> KMSDLRTVTLYKGKAGFGFSLLGP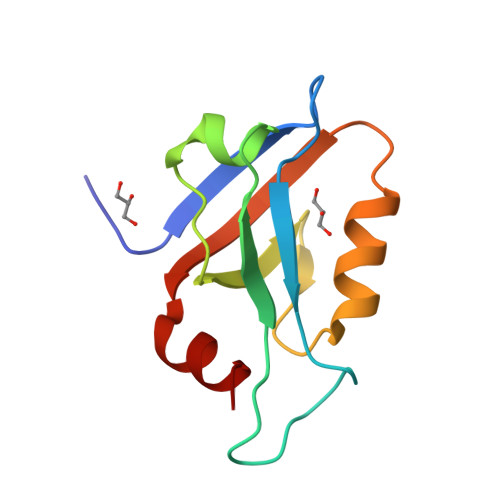AKAGPAEEGEPVGIFISRILPEGAAIESGQVFEGDQILSMNGQDLALASYRQAANLVKHITDGVMTLNLTANPGMYDLYKQ>[3x]MAHHHHHHMFEFDGKVAVITGAGSGFGRAFAEKGASLGMKLVLADVDEGALARTVDTLRAAGAEVIGVRTDVSNGAQVQALADAALEAFGKVHLLFNNAGVGAGGFLWESSANDWAWVFGVNVMGVAHGVRVFAPIMLGQNEAAHIVNTASVAGLLSPPSMGIYNASKHAVVSLTETLYHDLRNAGGEVGCSLLCPAFVPTGIADAERVRPEALRNEAQPTRS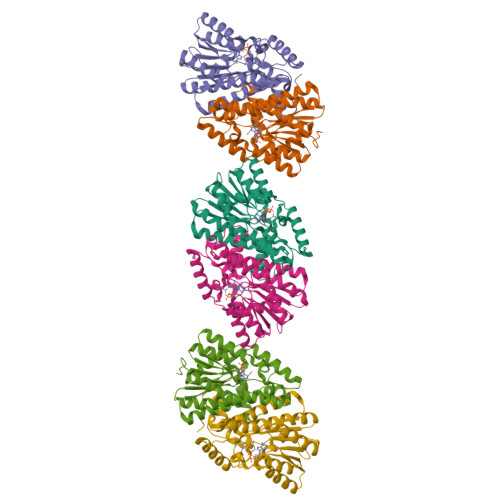QLAADRQLQRAVRSGKLGATDVATLTFEAIAERRFYILTHPAILATVRLRHEDIELQRNPTDPLSLKPEVKEAR> GSLEEM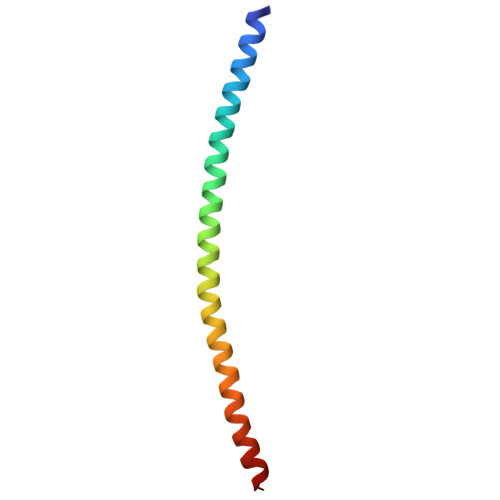QRRADQLADESLESTRRMLQLVEESKDAGIRTLVMLDEQGEQLDRVEEGMNHINQDMKEAEKNLKDLW> YVDVGPDSVKSACIEVDIQQTFFDKTWPRPIDVSKADGIIYPQGR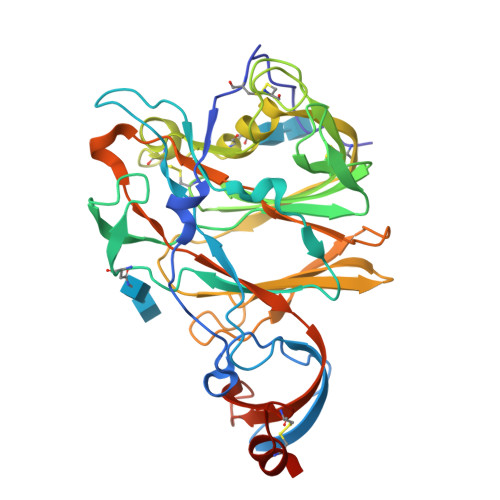TYSNITITYQGLFPYQGDHGDMYVYSAGHATGTTPQKLFVANYSQDVKQFANGFVVRIGAAANSTGTVIISPSTSATIRKIYPAFMLGSSVGNFSDGKMGRFFNHTLVLLPDGCGTLLRAFYCILEPRSGNHCPAGNSYTSFATYHTPATDCSDGNYNRNASLNSFKEYFNLRNCTFMYTYNITEDEILEWFGITQTAQGVHLFSSRYVDLYGGNMFQFATLPVYDTIKYYSIIPHSIRSIQSDRKAWAAFYVYKLQPLTFLLDFSVDGYIRRAIDCGFNDLSQLHCSYESHHHHHH>[3x]MAYSQGGGKKKVCYYYDGDIGNYYYGQGHPMKPHRIRMTHNLLLNYGLYRKMEIYRPHKATAEEMTKYHSDEYIKFLRSIRPDNMSEYSKQMQRFNVGEDCPVFDGLFEFCQLSTGGSVAGAVKLNRQQTDMAVNWA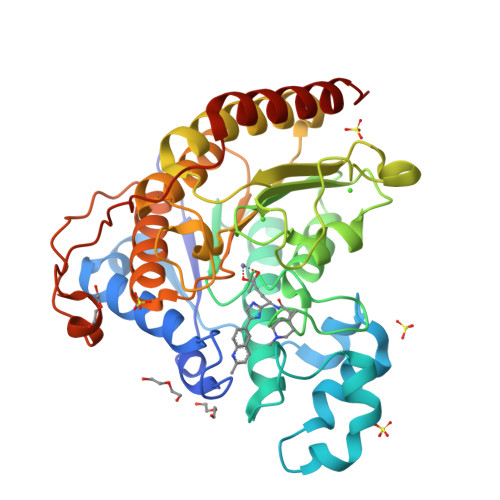GGLHHAKKSEASGFCYVNDIVLAILELLKYHQRVLYIDIDIHHGDGVEEAFYTTDRVMTVSFHKYGEYFPGTGDLRDIGAGKGKYYAVNFPMRDGIDDESYGQIFKPIISKVMEMYQPSAVVLQCGADSLSGDRLGCFNLTVKGHAKCVEVVKTFNLPLLMLGGGGYTIRNVARCWTYETAVALDCEIPNELPYNDYFEYFGPDFKLHISPSNMTNQNTPEYMEKIKQRLFENLRMLPH O-phosphoseryl-tRNASec:selenocysteinyl-tRNASec synthase (SepSecS; SEPSECS) is an ubiquitously expressed enzyme that catalyzes the terminal reaction of selenocysteine synthesis. SepSecS converts the phosphoseryl (Sep) group into the selenocysteinyl (Sec) moiety in a mechanism that requires selenocysteine tRNA (tRNASec) and a pyridoxal-5-phosphate (PLP) cofactor. Previous structural work has shown that SepSecS is an obligate tetramer held by interactions between two homodimers. Recently, two research groups reported that four distinct mutations in human SEPSECS caused congenital cerebellar atrophy termed pontocerebellar hypoplasia type 2D (PCH2D).

To establish whether mutations T325S and Y334C alter the structure of SepSecS, we solved crystal structures of holo T325S and the T325S-tRNASec and Y334C-tRNASec complexes. The binary complex crystals belonged to the trigonal space group and contained two SepSecS dimers and one tRNASec molecule in the asymmetric unit, whereas those of the holo T325S were of the orthorhombic space group with half of the SepSecS tetramer in the asymmetric unit. On the other hand, Thr325 is located in helix α12 and ~15Å away from the active site. We hypothesized that the insertion of Ser in position 325 could introduce a kink in α12, thereby altering both the orientation of PLP and the overall conformation of the active site in human SepSecS4. Inspection of the initial Fo-Fc electron density difference maps confirmed that Thr325 was substituted with Ser in the T325S variant and that Tyr334 was replaced with Cys in Y334C. A closer inspection of the crystal structure revealed that the Thr325 → Ser replacement does not cause any changes in the tetrameric structure of SepSecS. Based on these observations, we conclude that pathogenic mutations Thr325Ser and Tyr334Cys do not alter the three-dimensional structure of the SepSecS tetramer. The WT enzyme has a Tm value of 70.6 ± 1.0 °C. While the tetrameric T325S70 and Y334C70 have Tm values that are lower by ~5 °C with T325S70 having a Tm value of 65.0 ± 0.8 °C and Y334C70 having Tm of 64.6 °C ± 0.0 °C. In contrast, because only a small fraction of the T325S variant co-purifies with GroEL, it is likely the least damaging of the pathogenic variants. In contrast to the A239T variant, T325S contains a significant proportion of tetramers, and its fraction that co-elutes with GroEL is capable of adopting a tetrameric structure over time.

>[2x]MNRESFAAGERLVSPAYVRQGCEARRSHEHLIRLLLEKGKCPENGWDESTLELFLHELAIMDSNNFLGNCGVGEREGRVASALVARRHYRFIHGIGRSGDISAVQPKAAGSSLLNKITNSLVLDIIKLAGVHTVANCFVVPMATGMSLTLCFLTLRHKRPKAKYIIWPRIDQKSCFKSMITAGFEPVVIENVLEGDELRTDLKAVEAKVQELGPDCILCIHSTTSCFAPRVPDRLEELAVICANYDIPHIVNNAYGVQSSKCMHLIQQGARVGRIDAFVQSLDKNFMVPVGGAIIAGFNDSFIQEISKMYPGRASASPSLDVLISLLSLGSNGYKKLLKERKEMFSYLSNQIKKLSEAYNERLLHTPHNPISLAMTLKTLDEHRDKAVTQLGSMLFTRQVSGARVVPLGSMQTVSGYTFRGFMSHTNNYPCAYLNAASAIGMKMQDVDLFIKRLDRCLKAVRKERSKESDDNYDKTEDVDIEEMALKLDNVLLDTYQDASS>SAGIVPYQVKAQLYLFPGPEAELIRAAAEASLRDYISAQRRLGRDIRRSALFATLHVEGVQRVELQEPAA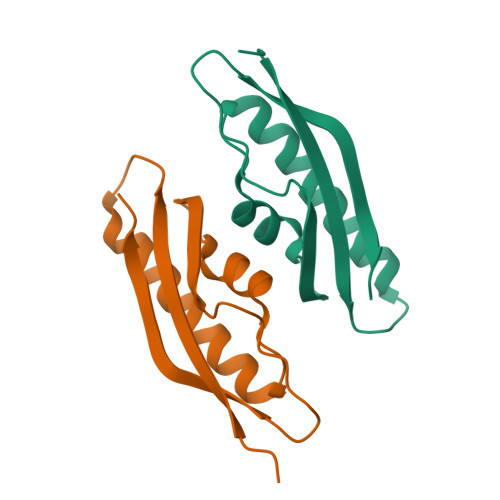DVVLDETQAAYCTGYAITLGGVDELEHHHHHH[2x]>[2x]MAEEVSNKQVILKNYVTGYPKESDMEIKNVTIKLKVPEGSNDVVVKNLYLSCDPYMRSRMRKIEGSYVESFAPGSPITGYGVAKVLESGD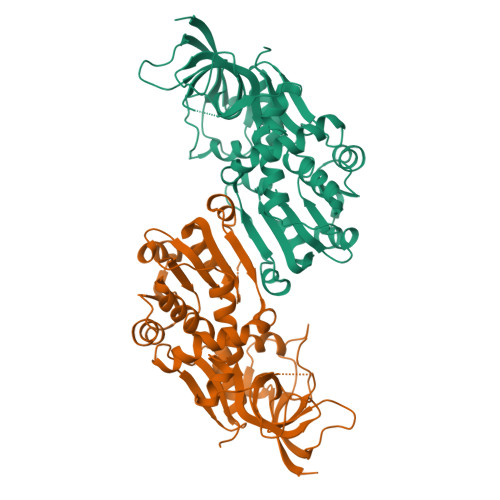PKFQKGDLVWGMTGWEEYSIITPTQTLFKIHDKDVPLSYYTGILGMPGMTAYAGFHEVCSPKKGETVFVSAASGAVGQLVGQFAKMLGCYVVGSAGSKEKVDLLKSKFGFDEAFNYKEEQDLSAALKRYFPDGIDIYFENVGGKMLDAVLVNMKLYGRIAVCGMISQYNLEQTEGVHNLFCLITKRIRMEGFLVFDYYHLYPKYLEMVIPQIKAGKVVYVEDVAHGLESAPTALVGLFSGRNIGKQVVMVSRELEHHHHHH>GSEELLDLFNRQVTQEFTASQVYLSASIWFDQNDWEGMAAYMLAESAEEREHGLGFVDFANKRNIPIELQAVPAPVSCAEWSSPEDVWQSILELEQANTRSLLNLAEAASTCHDFAVMAFLNPFHLQQVNEEDKIGSILAKVTDENRTPGLLRSLDVVSFLGPCLFRS[8x]

A novel ferritin was recently found in Pseudo-nitzschia multiseries (PmFTN), a marine pennate diatom that plays a major role in global primary production and carbon sequestration into the deep ocean. Ferritin is a 24-mer that forms a hollow sphere, takes up soluble ferrous iron, oxidizes it at di-iron ferroxidase centers, and stores the iron oxide mineral in its central cavity. Sites A and B comprise the conserved ferroxidase active site, and site C forms a pathway leading toward the central cavity where iron storage occurs. The structures confirm the typical ferritin arrangement: 24 subunits assemble to form a hollow spherical shell.

Zn (1 h)refers to the structure of PmFTN from crystals soaked in Zn(II) for 1 h. Zinc ions are competitive inhibitors of ferritin and bacterioferritin. Crystal structures of Zn(II)-inhibited ferritin confirm that this metal binds to the ferroxidase site and site C. The zinc ions are coordinated by the same residues as seen in the structures from aerobically iron-soaked crystals. Glu-130 is predominately coordinated to the zinc ion in site C, although in three of the monomers of the asymmetric unit, Glu-130 adopts two equal occupancy conformations, one that coordinates to the zinc ion in site B, and the other that coordinates to the zinc ion in site C. Furthermore, the zinc ion at site A is modeled as coordinated by two water molecules, one of which is bridging to site B. This arrangement of coordinated solvent is similar to that observed in the iron-soaked structures. An overlay of the zinc structure with the iron structures showed that the zinc atom in site B is slightly shifted toward site A and that the zinc atom in site C is closer toward the core as compared with the iron. Zn(II) bound to sites A, B, and C in contrast to the two sites observed in EcFtnA. Furthermore, overall Zn(II) occupancy of the three metal sites resembles iron bound in the presence of dioxygen in PmFTN rather than mimicking Fe(II) binding. Thus, the use of Zn(II) and likely other metal ions as analogs of Fe(II)/Fe(III) may not identify the correct binding sites in other ferritins.>GLEAVRKRPGMYIGSTSERGLHHLVWEIVDNSIDEALAGYANQIEVVIEKDNWIKVTDNGRGIPVDIQEKMGRPAVEVILTSSVVNALSQDLEVYVHRNETIYHQAYKKGVPQFDLKEVGTTDKTGTV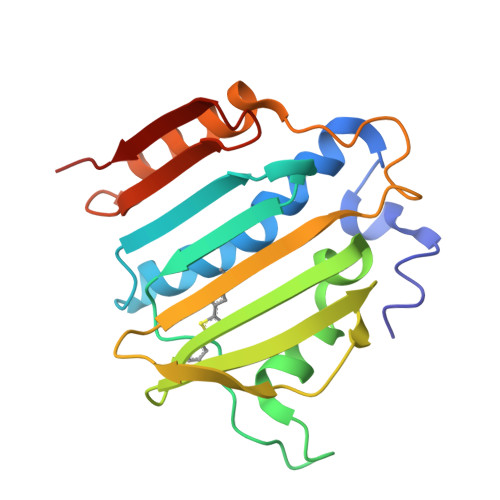IRFKADGEIFTETTVYNYETLQQRIRELAFLNKGIQITLRDERDEENVREDSYHYE[2x]>MERNHWNEKSSGAKRSRERDLTLSTIRSILAADERLRIKASSYLGVGRGVDDEAVIDIFPTGQTMSFLRLLHGFLGTCRGQSMHQVLRDPCVLRKQLLYGVCKTLFDTITVRRVAEEWKLHAALFPYRALDEEDLEQYLLVWSASLRQSVQTGVLGALRDILYQYADNDDYGLYVDWCVTVGLVPLLDVKTKPSEAAERAQFVRAAVQRATETHPLAQDLLQANLALLLQVAERLGAVRVANAPEVRVFKKVRSERLEAQLRGKHIRLYVAAEPLAYERDKLLFTTPVAHLHEEILRYDGLCRHQKICQLLNTFPVKVVTASRHELNCKKLVEMMEQHDRGSDAKKSIMKFLLNVSDSKSRIGIEDSVESFLQDLTPSLVDQNRLLPARGPGGPGVVGPGGAVVGGPAGHVGLLPPPPGPAAPERDIRDLFKKQVIKCLEEQIQSQVDEIQDLRTLNQTWENRVRELRDLLTRYASRREDSMSLGARDAELYHLPVLEAVRKARDAAPFRPLAVEDNRLVANSFFSQFVPGTESLE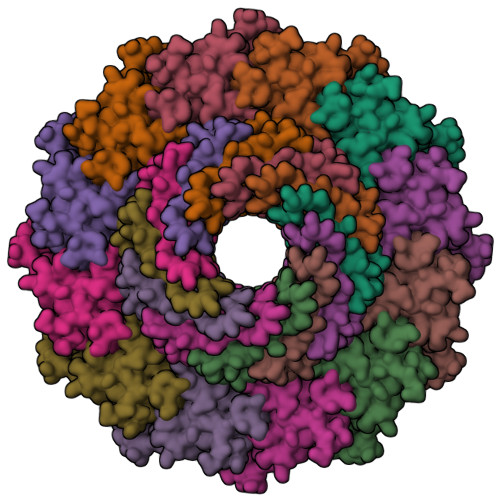RFLTQLWENEYFRTFRLRRLVTHQGAEEAIVYSNYTVERVTLPYLCHILALGTLDPVPEAYLQLSFGEIVAAAYDDSKFCRYVELICSREKARRRQMSREAAGGVPERGTASSGGPGTLERSAPRRLITADEERRGPERVGRFRNGGPDDPRRAGGPYGFH[12x]>GSAPSEITRAGILQAIAEHDRIGPEAFRATYGFHAATSYFLEHEGRLYDSKAIAGVAHMYDFGVALKPSSPGLSGGLKHAVAWLRREGFTIREAPKTFHRRVGDVRPARRAMGPALHRPVLLLWAIGQAVARAPRLQPWSTTRDAVAPLMEKYGQVEDGVDGVRYPFWALVRDDLWCVEQAEELTLTSRGRRPTLESLNAVDPSAGLREDDYNLLRSQPEAAASAAAGLIARYFHLLPAGLLEDFGLHELLAGRWPDALRPLLGETFKDRDAIWRAYGGQKMAGIGCLADGILSAFSDDKGPYADGRIPDTTWIAYVGDGLSGDQKLTDGNELMAEHQAVGRALRYWHKPFQGQWSFETWAVIVQRRLRWGLGEDKLPRREFLWVLAPVPSPERETWPPEVLEALEADTGELHDDTGDYRPSDLALTPGAPDGTESDDEAYRRLAQKAEANAERRGQLKKPTVADKYVRDPSARGAVLKRCQKRCENPECAGHP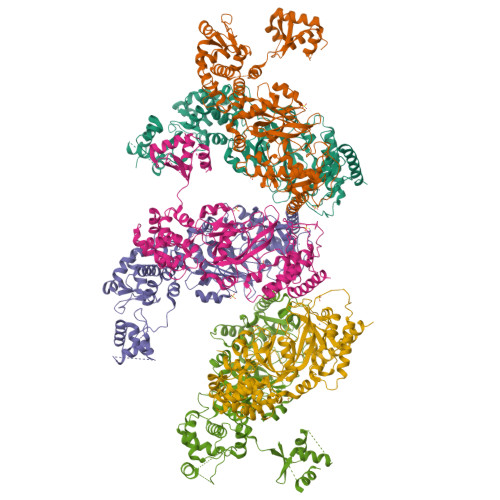TELTKAGLPILQVDHVNDLAKGGPDVPWNMIALCPNCHALKTYGANKVRLQRLLAATARRLHEEKLQ[6x]> AQIVKLGGDDGSLAFVPSKISVAAGEAIEFVNNAGFPHNIVF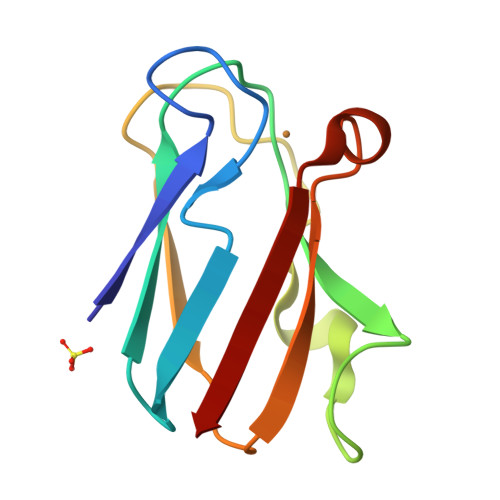DEDAVPAGVDADAISYDDYLNSKGETVVRKLSTPGVYGVYCEPHAGAGMKMTITVQ> MNYSQIERMARKGVAFFTDPSRPMNLIKQGEYGYDENGFEIPPMEQVIPISGATRRPNAREIDGETIRASDILGIFNNDHEINEGDYIEIDGIRHVVV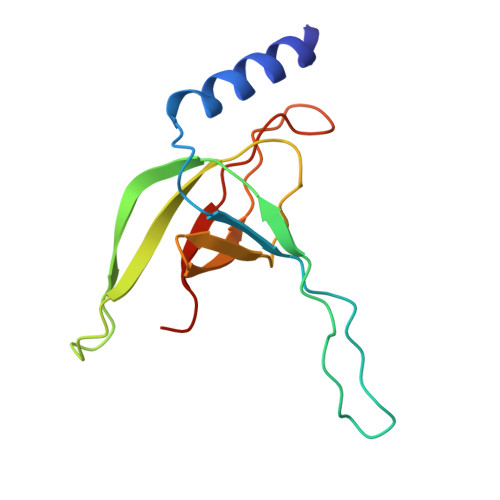DARPVQASLEPVAYRPVLRRVSVGG> TPAITLENPDIKYPLRLIDKEVVNHDTRRFRFALPS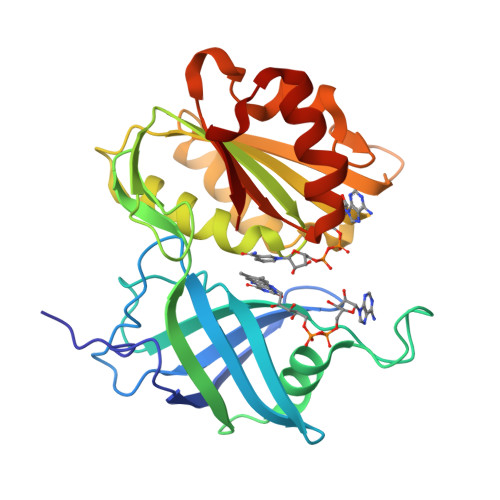PEHILGLPVGQHIYLSARIDGNLVIRPYTPVSSDDDKGFVDLVIKVYFKDTHPKFPAGGKMSQYLESMKIGDTIEFRGPNGLLVYQGKGKFAIRPDKKSSPVIKTVKSVGMIAGGTGITPMLQVIRAIMKDPDDHTVCHLLFANQTEKDILLRPELEELRNEHSARFKLWYTVDRAPEAWDYSQGFVNEEMIRDHLPPPEEEPLVLMCGPPPMIQYACLPNLERVGHPKERCFAF>STAGKVIKCKAAVLWEVKKPFSIEDVEVAPPKAYEVRIKMVAVGICHTDDHVVSGNLVTPLPVILGHEAAGIVESVGEGVTTVKPGDKVIPLFTPQCGKCRVCKNPESNYCLKNDLGNPRGTLQDGTRRFTCRGKPIHHFL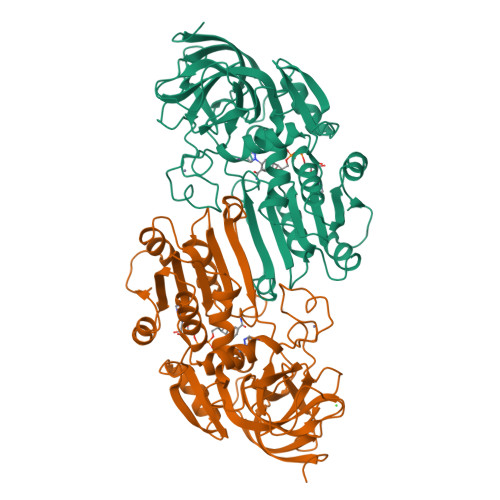GTSTFSQYTVVDENAVAKIDAASPLEKVCLIGCGFSTGYGSAVNVAKVTPGSTCAVFGLGGVGLSAVMGCKAAGAARIIAVDINKDKFAKAKELGATECINPQDYKKPIQEVLKEMTDGGVDFSFEVIGRLDTMMASLLCCHEACGTSVIVGVPPASQNLSINPMLLLTGRTWKGAVYGGFKSKEGIPKLVADFMAKKFSLDALITHVLPFEKINEGFDLLHSGKSIRTVLTF[2x]5-bromo-7-{5-[(3-{[(4-tert-butylphenyl)carbamoyl]amino}propyl)(propan-2-yl)amino]-5-deoxy-beta-D-ribofuranosyl}-7H-pyrrolo[2,3-d]pyrimidin-4-amine | C28 H40 Br 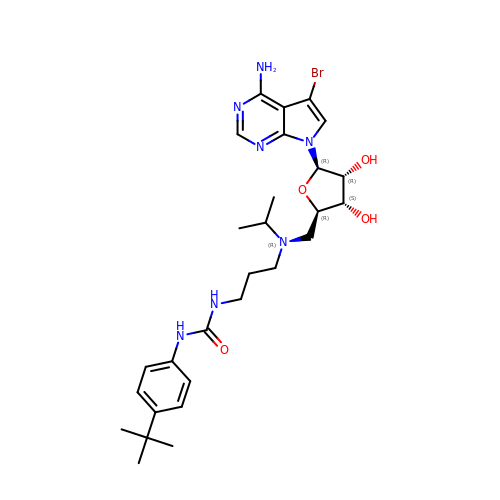N7 O4 | IQCKJUKAQJINMK-HUBRGWSESA-N> MKIAVIGQSLFGQEVYKELKNEGHMIVGVFTIPDKDGKVDPLAIEAEKDGVPVFKFPRWRLKGKAITEVVDQYKAVGAELNVLPFCSQFIPMEVIDHPKHGSIIYHPSLLPRHRGASAINWTLIHGDKKGGFTVFWADDGLDTGPILLQRECDVEPNDNVNSIYKRFLFPEGVKGMVEAVRLIATGKAPRIKQPEEGATYECIQKKENSKIDWNQPAEAIHNWIRGNDRVPGAWAEIDGKSVSFYGSTLLENDHFSSNGQPLEIPGASRAALVTKNGLVLFGNDGKMLLVKNLQFEDGKMIPGSQYFKAGVEHHHHHH

10-Formyltetrahydrofolate dehydrogenase (FDH), which is composed of a small N-terminal domain (Nt-FDH) and a large C-terminal domain, is an abundant folate enzyme in the liver and converts 10-formyltetrahydrofolate (10-FTHF) to tetrahydrofolate (THF) and CO2. Nt-FDH alone possesses a hydrolase activity, which converts 10-FTHF to THF and formate in the presence of β-mercaptoethanol. The N-terminal hydrolase domain of FDH (Nt-FDH) binds folate and is homologous to glycinamide ribonucleotide formyltransferase (GART) and methionyl-tRNA formyltransferase (FMT), enzymes that are crucial for de novo purine biosynthesis and translation initiation, respectively. In this study, we determined crystal structures of zebrafish wild-type apo Nt-FDH (zNt-FDH) and its ternary complexes with the substrate 10-formyl-5,8-dideazafolate (10-FDDF) and the products tetrahydrofolate (THF) and formate.

In the active site, the formyl group of the substrate is converted into the product formate during catalysis. In the structure of the formate complex, the formate molecule interacts with His106 and Asp142. The O1 atom of formate is directly hydrogen-bonded to OD2 of Asp142 (within 2.73 Å). The O1 atom of the formate interacts with the ND1 atom of His106 and the OD1 atom of Asp142 at distances of 3.46 and 3.19 Å, respectively. A hypothesis has been proposed in which β-mercaptoethanol is required for replacing and releasing the product from the catalytic site because of the structural similarity between β-mercaptoethanol and the product formate.> SNAGGSSPITGLVYDQRMMLHHNMWDSHHPELPQRISRIFSRHEELRLLSRCHRIPARLATEEELALCHSSKHISIIKSSEHMKPRDLNRLGDEYNSIFISNESYTCALLAAGSCFNSAQAILTGQVRNAVAIVRPPGHHAEKDTACGFCFFNTAALTARYAQSITRESLRVLIVDWDVHHGNGTQHIFEEDDSVLYISLHRYEDGAFFPNSEDANYDKVGLGKGRGYNVNIPWNGGKMGDPEYMAAFHHLVMPIAREFAPELVLVSAGFDAARGDPLGGFQVTPEGYAHLTHQLMSLAAGRVLIILEGGYNLTSISESMSMCTSMLLGDSPPSLDHLTPLKTSATVSINNVLRAHAPFWSSLR

While Sirt2 features an NAD+-dependent catalytic mechanism and belongs to class III HDACs, also referred to as sirtuins, HDAC6 is a Zn2+-dependent lysine deacylase and has been classified as a class IIb HDAC. Although both deacylases are classified as histone deacetylases, they share acetylated α-tubulin (α-tubulin K40ac) as their major substrate and are hence frequently referred to as tubulin deacetylases. Three new crystal structures of Sirt2 and HDAC6, respectively, in complex with Sirt2- or HDAC6-targeted building blocks, provided structural evidence for the interaction of our dual Sirt2/HDAC6 inhibitors with both targets.

To obtain structural insights into the HDAC6 binding modes of the dual Sirt2/HDAC6 inhibitors 32 and 33, we submitted 55 and 57, which represent the HDAC6-targeted subunits of 32 and 33, respectively, for crystallization trials with HDAC6. As the crystal structures of human and zebrafish CD2 enzymes are essentially identical, the zebrafish HDAC6 CD2 (henceforth simply “HDAC6”) serves as a more readily studied surrogate of the human enzyme. The HDAC6–55 complex crystallized in space group P21 with one monomer in the asymmetric unit. The hydroxamate N–O– group coordinates to the catalytic Zn2+ ion with a Zn2+–O separation of 2.0 Å. The hydroxamate C=O group accepts a hydrogen bond from the Zn2+-bound water molecule, which also forms hydrogen bonds with the imidazole side chains of H573 and H574. Additionally, the phenolic hydroxyl group of Y745 forms poorly oriented hydrogen bonds with the hydroxamate C=O and NH groups. The phenyl subunit of 55 is sandwiched between F583 and F643, making staggered π-stacking interactions. The carbonyl of the inhibitor capping group accepts a hydrogen bond from a nearby water molecule and is positioned 3.6 Å away from a molecule of ethylene glycol. The acetamide NH group of the inhibitor capping group is 3.7 Å from the side chain of S531 and the acetamide methyl group is oriented toward solvent, although electron density coverage is poor in this region of the electron density map.> TSR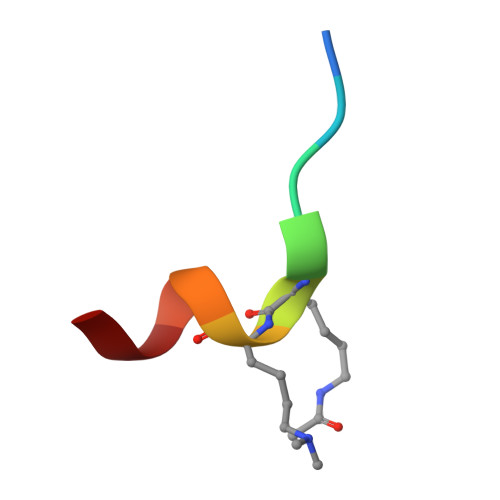HKKLMFK> MNHKVHHHHHHHHMLETLINKIYTGPLGEELVQTLYLRIWAMEETPESLKILQMREDIRDQVLKMKTERWLRTLIRGEKTKLKDFQKRYEEVHPYLMKEKVEQVIMEEAWSLAAHIV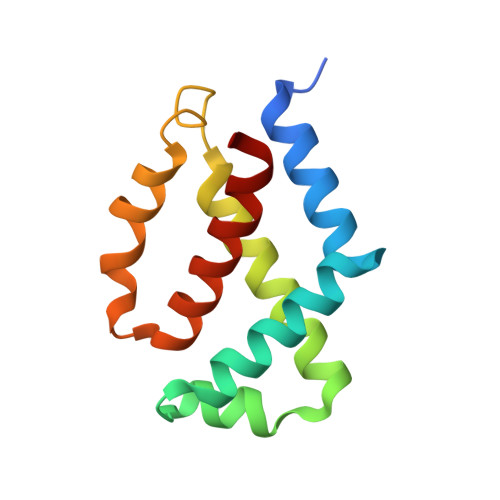QE> GMADEATRRVVSEIPVLKTNAGPRDRELWVQRLKEEYQSLIRYVENNKNADNDWFRLESNKEGTRWFGKCWYIHDLLKYEFDIEFDIPITYPTTAPEIAVPE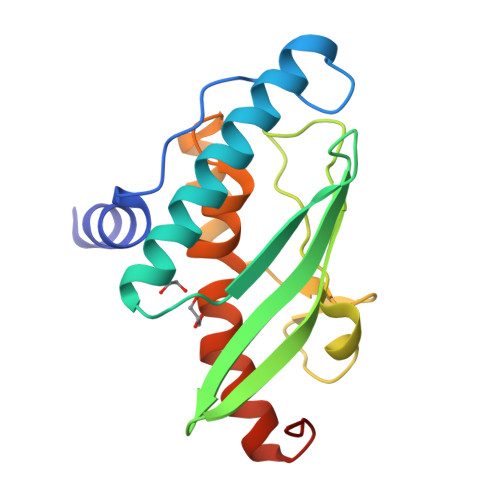LDGKTAKMARGGKICLTDHAKPLWARNVPKFGLAHLMALGLGPWLAVEIPDLIQKGVIQHKEKCNQ>[3x]MDLADRFAELERRYDARLGVYVPATGTTAAIEYRADERFAFCATFKAPLVAAVLHQNPLTHLDKLITYTSDDIRSISPVAQQHVQTGMTIGQLCDAAIRYSDGTAANLLLADLGGPGGGTAAFTGYLRSLGDTVSRLDAEEPELNRDPPGDERDTTTPHAIALVLQQLVLGNALPPDKRALLTDWMARNTT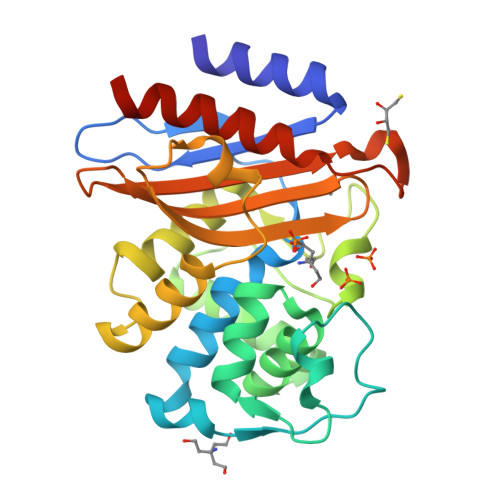GAKRIRAGFPADWKVIDKTGTGDYGRANDIAVVWSPTGVPYVVAVMSDRAGGGYDAEPREALLAEAATCVAGVLALEHHHHHH;> GGGGGG>AMATRGANVIWFRHGLRLHDNPALLAALADKDQGIALIPVFIFDGESAGTKNVGYNRMRFLLDSLQDIDDQLQAATDGRGRLLVFEGEPAYIFRRLHEQVRLHRICIEQDCEPIWNERDESIRSLCRELNIDFVEKVSHTLWDPQLVIETNGGIPPLTYQMFLHTVQIIGLPPRPTADARLEDATFVELDPEFCRSLKLFEQLPTPEHFNVYGDNMGFLAKINWRGGETQALLLLDERLKVEQHAFERGFYLPNQALPNIHDSPKSMSAHLRFGCLSVRRFYWSVHDLFKNVQLGVQMTGGAHITGQLIWREYFYTMSVNNPNYDRMEGNDICLSIPWAKPNENLLQSWRLGQTGFPLIDGAMRQLLAEGWLHHTLRNTVATFLTRGGLWQSWEHGLQHFLKYLLDADWSVCAGNWMWVSSSAFERLLDSSLVTCPVALAKRLDPDGTYIKQYVPELMNVPKE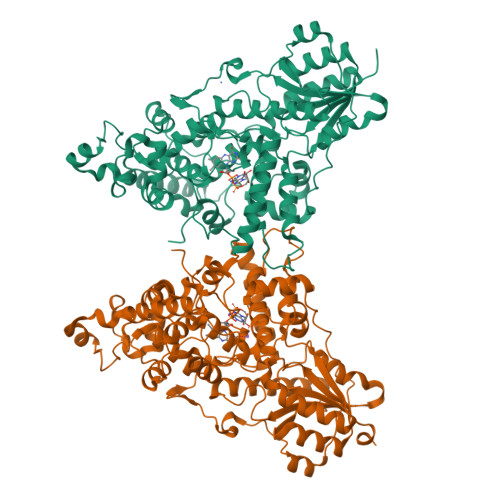FVHEPWRMSAEQQEQYECLIGVHYPERIIDLSMAVKRNMLAMKSLRNSLITPPPHCRPSNEEEVRQFFWLADV[2x]3-(3-chlorophenyl)-N-{2-[2-(1H-imidazol-1-yl)pyrimidin-4-yl]ethyl}propan-1-amine | C18 H20 Cl N5 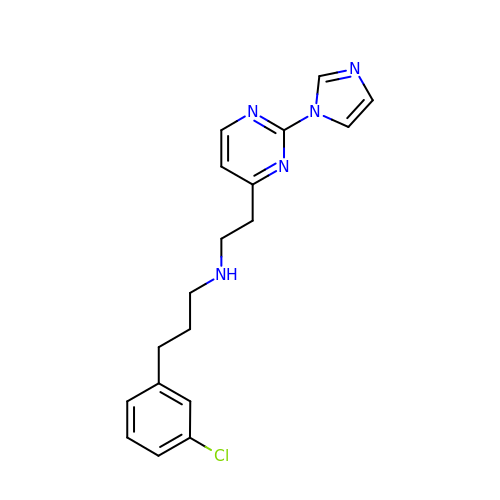| VPDCBONBBAYCIG-UHFFFAOYSA-N>[2x]CGC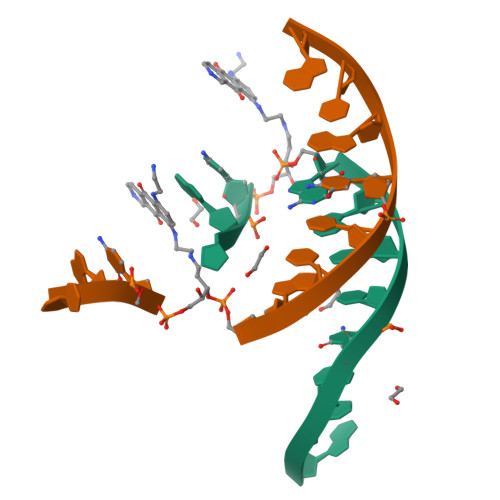XAATTCGCG> MRGSHHHHHHTDLRADKASSIELKFDRNKGEVGDILIGTVRINNIKNFAGFQVNIVYDPKVLMAVDPETGKEFTSSTFPPGRTVLKNNAYGPIQIADN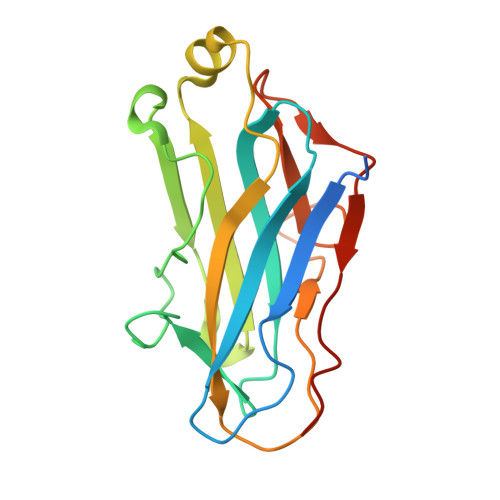DPEKGILNFALAYSYIAGYKETGVAEESGIIAKIGFKILQKKSTAVKFQDTLSMPGAISGTQLFDWDGEVITGYEVIQPDVLSLGDEPF> PAAEGSGE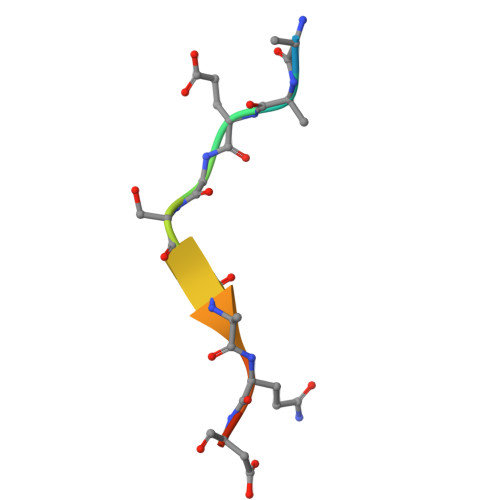QDFT>GAHMVTSNVVLVSGEGERFTVDKKIAERSLLLKNYLNDMGDDDDEDDDEIVMPVPNVRSSVLQKVIEWAEHHRDSNFPDEDDDDSRKSAPVDSWDREFLKVDQEMLYEIILAANYLNIKPLLDAGCKVVAEMIRGRSPEEIRRTFNIVNDFTPEEEAAIRRENEWAEDR[2x];>[2x]GAGTLIKDNLKRDLITSLPFEISLKIFNYLQFEDIINSLGVSQNWNKIIRKSTSLWKKLLISENFVSPKGFNSLNLKLSQKYPKLSQQDRLRLSFLENIFILKNWYNPKFVPQRTTLRGHMTSVITCLQFEDNYVITGADDKMIRVYDSINKKFLLQLSGHDGGVWALKYAHGGILVSGSTDRTVRVWDIKKGCCTHVFEGHNSTVRCLDIVEYKNIKYIVTGSRDNTLHVWKLPKESSVPDHGEEHDYPLVFHTPEENPYFVGVLRGHMASVRTVSGHGNIVVSGSYDNTLIVWDVAQMKCLYILSGHTDRIYSTIYDHERKRCISASMDTTIRIWDLENGELMYTLQGHTALVGLLRLSDKFLVSAAADGSIRGWDANDYSRKFSYHHTNLSAITTFYVSDNILVSGSENQFNIYNL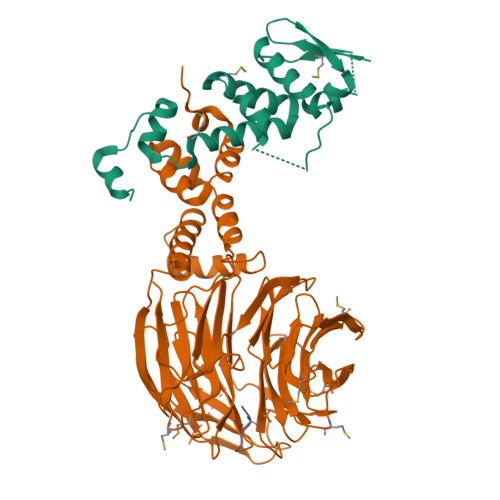RSGKLVHANILKDADQIWSVNFKGKTLVAAVEKDGQSFLEILDFS;>GLLTPPQSG[2x]> IVGGYECKAYSQPHQVSLN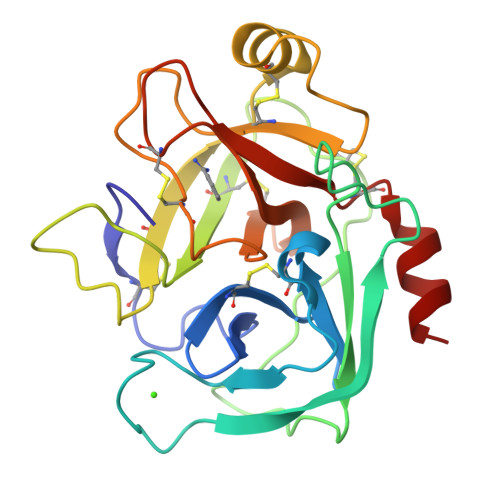SGYHFCGGSLVNENWVVSAAHCYKSRVEVRLGEHNIKVTEGSEQFISSSRVIRHPNYSSYNIDNDIMLIKLSKSATLNTYVQPVALPSSCAPAGTMCTVSGWGNTMSSTADKNKLQCLNIPILSYSDCNNSYPGMITNAMFCAGYLEGGKDSCQGDSGGPVVCNGELQGVVSWGYGCAEPGNPGVYAKVCIFNDWLTSTMA> TTHFVIIDRDGTVVSSTNTLSNFFGTGKYTAGFFLNNQLQNFGSEGFNSYEPGKRSRTFMAPTVLKKDGETIGIGSPGGNRIPQILTPILDKYTHGKGSLQDIINEYRFTFEKNTAYTEIQLSSEVKNELSRKGLNVKKKVSPAFFGGVQALIKDERDNVI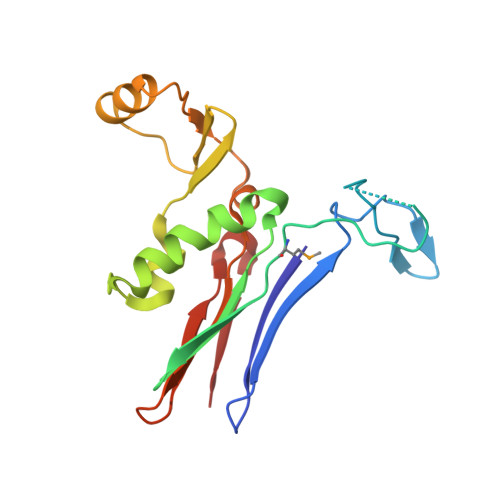TGAGDGRRNGTWKSNK>[2x]SLNTDDIQGDILVGMHKQKQLFYFFAINDPATFKTHLASDIAPVVASVTQLSNVAT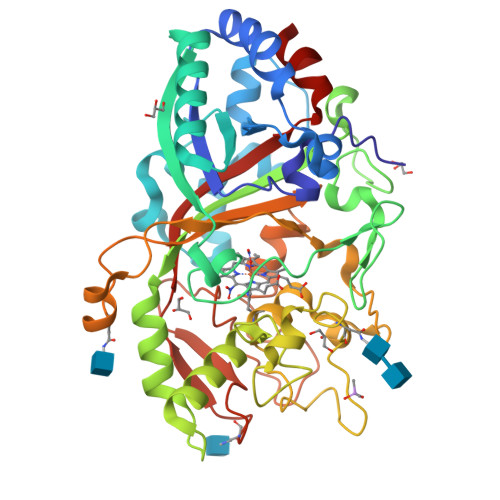QPLVALNIAFSNTGLLALGVTDNLGDSLFANGQAKDATSFKESTSSWVPQFAGTGIHGVIILASDTTDLIDQQVASIESTFGSSISKLYSLSASIRPGNEAGHEMFGFLDGIAQPAINGFNTPLPGQNIVDAGVIITGATNDPITRPSWAVGGSFLAFRQLEQLVPEFNKYLLDNAPAGSGSLQARADLLGARMVGRWKSGAPIDLTPTADDPALGADAQRNNNFTYSHAGFDLGSDQSHCPFSAHIRKTRPRADLGGSLTPPNLSAGANSIMRSGIPYGPEVTSAESASNTTTQERGLAFVAYQAQLSQGFHFLQQTWADNANFPPGKTPATVGLDPIIGQNNGQPRVVNGLLPSNSSASLSIPQFVVSHGGEYFFSPPISAIGGRLSA> MAQNITARIGEPLVLKCKGAPKKPPQRLEWKLNTGRTEAWKVLSPQGGGPWDSVARVLPNGSLFLPAVGIQDEGIFRCQAMNRNGKETKSNYRVRVYQIPGKPEIVDSASELTAGVPNKVGTCVSEGSYPAGTLSWHLDGKPLVPNEKGVSVKEQTRRHPETG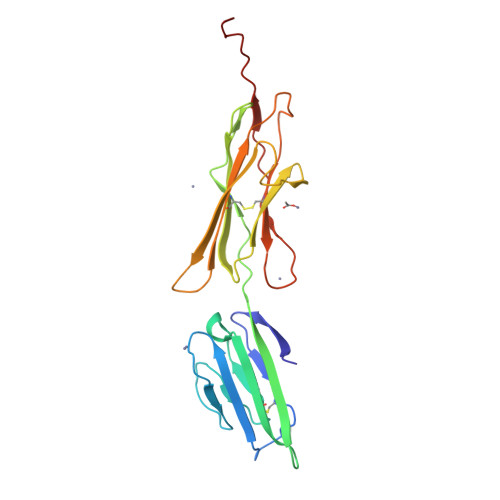LFTLQSELMVTPARGGDPRPTFSCSFSPGLPRHRALRTAPIQPRVWEPVPLEEVQL> MDHHHHHHNPCEKHSCIAVIDAGSTGSRLHIYSYDTDDTNTPIHIEEIWNKKIKPGFASIQPNSVTIDAYLTMLLADAPIHNIPVYFYATAGMRLLPQSQQKKYYDELDYWFRQQSQWQLVEAKTITGNDEALFDWLAVNYKLDTLKSVQNKSVGVMDMGGASVQIVFPMPKNAEISKHNQVELNI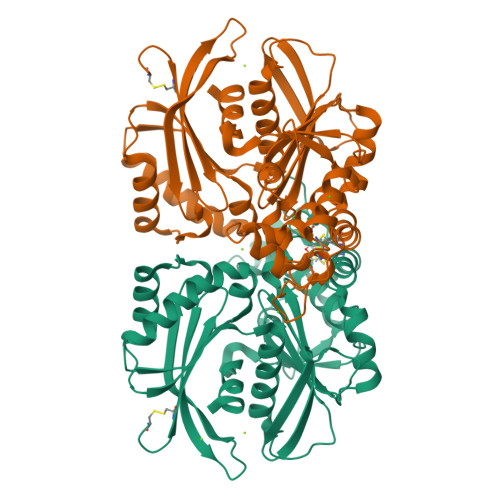YGQNINLYVHSFLGLGQTEMSHQFLNSPSCFANDYPLPDGESGQGNAPSCKEEVTSLMNSVHKVNQQIQPLLALNPVNEWYSIGGISNLASSQLFHFENSELTNQSLLQQGDNQICHQQWDILNGQYPDDEYLYQYCLLSSYYYALMVDGYGINPNQTIHYIPPEQNLDWTIGVVLHRA> MSFVITNPEALTVAATEVRRIRDRAIQSDAQVAPMTTAVRPPAADLVSEKAATFLVEYARKYRQTIAAAAVVLEEFAHALTT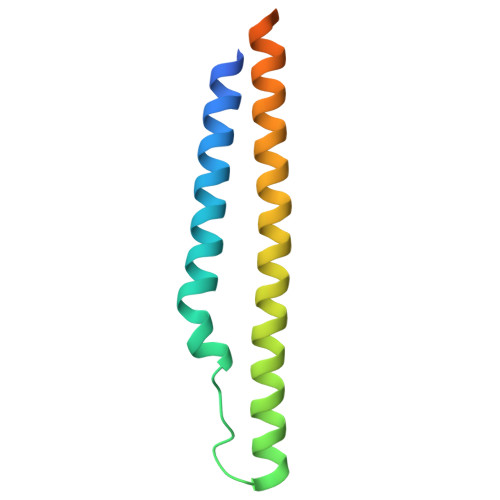GADKYATAEADNIKTFSSGETHHHHHH>[2x]MAPKAKIVLVGSGMIGGVMATLIVQKNLGDVVMFDIVKNMPHGKALDTSHTNVMAYSNCKVSGSNTYDDLKDADVVIVTAGFTKAPGKSDKEWNRDDLLPLNNKIMIEIGGHIKNNCPNAFIIVVTNPVDVMVQLLHQHSGVPKNKIVGLGGVLDTSRLKYYISQKLNVCPRDVNA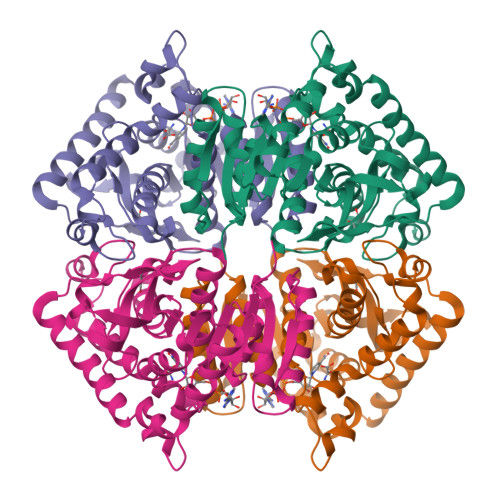HIVGAHGNKMVLLKRYITVGGIPLQEFINNKKITDQELDAIFDRTINTALEIVNLHASPYVAPAAAIIEMAESYIRDLRKVLICSTLLEGQYGHKDIFAGTPLVIGGNGVEQVIELQLNADEKKKFDEAVAETSRMKALIHHHHHH> MSLADDHIYVTSSGGSFLENVRKHMAEPFEKQSGVKVTLVPGTNPAHALKILSSRGTPPYDVAAFGGNDMYRLIRAKKLAQVDEKSVPSLADV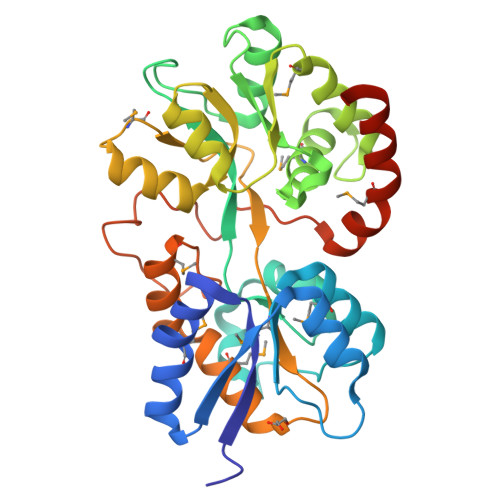PEKFKADWEGCGSLYDYSSVGIAYRPDKIQGGVKSWKEFVERTVAGEFGKQVFFNNLSSNVRGAEVLSMFGKIYGSGYGDIEASIATLERMKPHIFKFFTAFNDPVVLLTSGEGAIGPGWDGRTFIAEDSTKGMVKWVDPTEGAVSSGPVMAVVKGGKEDLAKAFMNYALGEEAQKAFCEAMYYGAVNRKVQYSEKLKHRLPSIDSVQLVDTALLIKNMSALLDLWNKRIASEGHHHHHH ethyl 5-{[(1R)-1-(ethoxycarbonyl)-2-oxopropyl]sulfanyl}-1,2-dihydro[1,2,3]triazolo[1,5-a]quinazoline-3-carboxylate 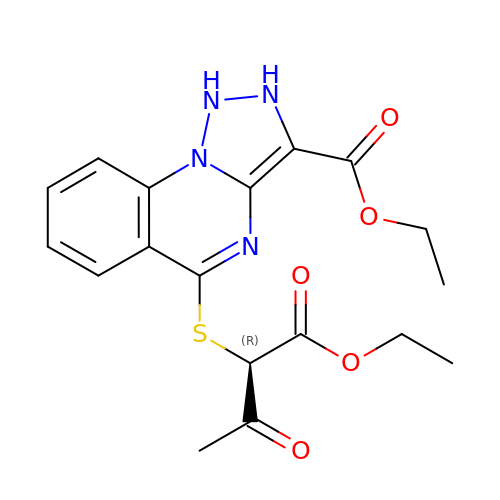| C18 H20 N4 O5 S | JTPUHTLSVQEMRB-CQSZACIVSA-N> YV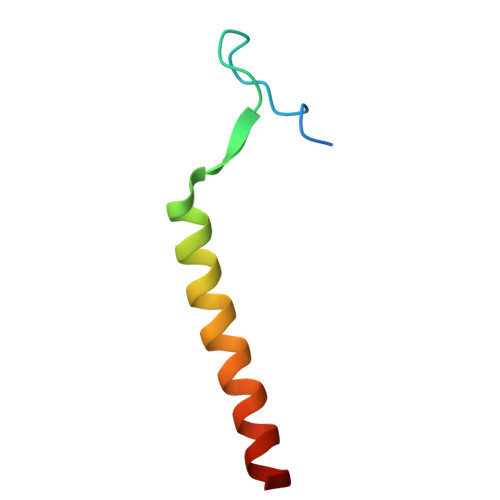ATRDNCCILDERFGSYCPTTCGIADFLNNYQTSVDKDLRTLEGILY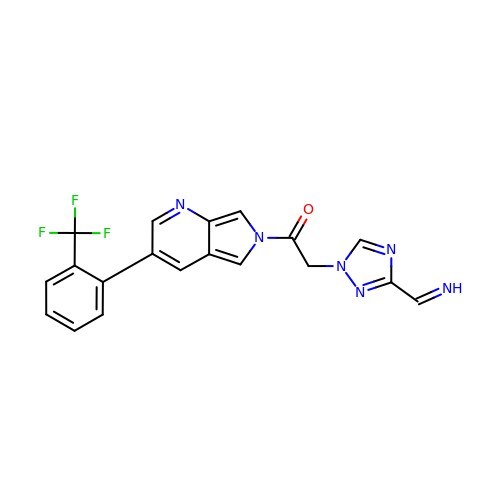2-{3-[(Z)-iminomethyl]-1H-1,2,4-triazol-1-yl}-1-{(3M)-3-[2-(trifluoromethyl)phenyl]-6H-pyrrolo[3,4-b]pyridin-6-yl}ethan-1-one | C19 H13 F3 N6 O | CZMOUVMERVDBNS-OUBWWKSTSA-N> MGACGSKGSTSDKGLASDKDGKKAKDRKEAWERIRQAIPREKTAEAKQRRIELFKKFDKNETGKLCYDEVYSGCLEVLKLDEFTSRVRDITKRAFDKSRTLGSKLENKGSEDFVEFLEFRLMLC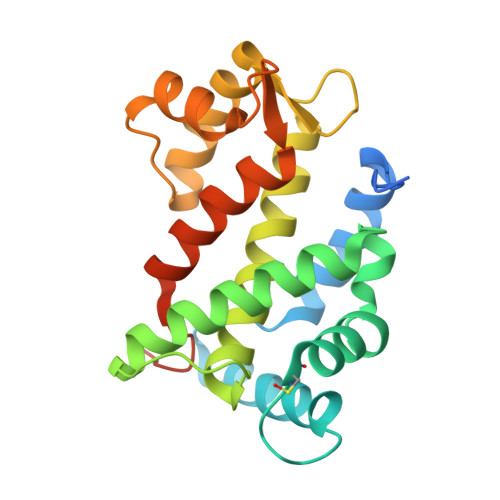YIYDFFELTVMFDEIDASGNMLVDEEEFKRAVPKLEAWGAKVEDPAALFKELDKNGTGSVTFDEFAAWASAVKLDADGDPDNVPESALEHHHHHH>[4x]MSGRLTGKVALVSGGARGMGASHVRAMVAEGAKVVFGDILDEEGKAMAAELADAARYVHLDVTQPAQWKAAVDTAVTAFGGLHVLVNNAGILNIGTIEDYALTEWQRILDVNLTGVFLGIRAVVKPMKEAGRGSIINISSIEGLAGTVACHGYTATKFAVRGLTKSTALELGPSGIRVNSIHPGLVK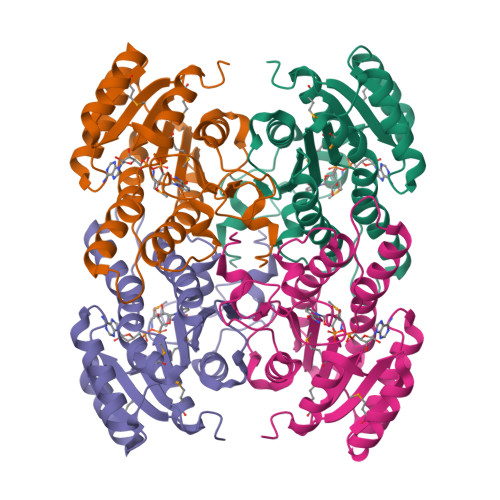TPMTDWVPEDIFQTALGRAAEPVEVSNLVVYLASDESSYSTGAEFVVDGGTVAGLAHNDFGAVEVSSQPEWVT>GPGSSMKYVSTRGEAPVLGFSDALLAGLARDGGLYLPQEYPQFTAEQIRALRGKSYV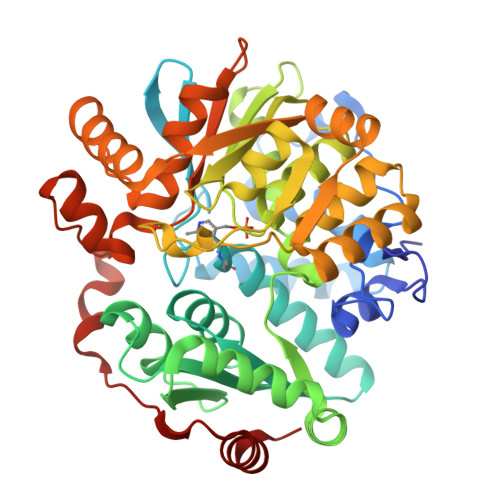EVALAVLTPFTGGEIPAADFERMVREAYGTFRHDAVCPLVQTDANEFVLELFHGPTLAFKDVAMQLLARMMDYVLAQRGERATIVGATSGDTGGAAIEAFGGRDNTDIFILFPNGRVSPVQQRQMTSSGFSNVHALSIEGNFDDCQNLVKGMFNDLEFCDALSLSGVNSINWARIMPQVVYYFTAALSLGAPDRAVSFTVPTGNFGDIFAGYVAKRMGLPIEQLIIATNDNDILSRTLESGAYEMRGVAQTTSPSMDIQISSNFERLLFEAHGRDAAAVRGLMQGLKQSGGFTISEKPLSAIRSEFSAGRSTVDETAATIESVLSKDGYLLDPHSAIGVKVAREKASGTAPMVVLATAHPAKFPDAVKAACGVEPQLPAWLCDLMQRKESFTVLHNELKIVEEYVRHHSRA[2x]Aureos typically consist of an N-terminal domain with unknown function, a basic region leucine zipper (bZIP) DNA-binding domain, and a C-terminal light-oxygen-voltage (LOV) sensing domain. LOV domains are a subgroup of the Per-Arnt-Sim (PAS) superfamily that sense blue light using a noncovalently bound flavin cofactor. Photon absorption of the flavin results in formation of a flavin-C4(a)-cysteinyl adduct with a conserved cysteine residue, which initiates a cascade of structural rearrangements within the LOV core that are propagated to the domain boundaries. Here, we present crystal structures of a fully light-adapted LOV dimer as well as of a dark state LOV monomer of PtAu1a.

To obtain the structure of a fully light-adapted PtAu1aLOV dimer, we set up crystallization screens of wildtype PtAu1aLOV under continuous blue light illumination and obtained colorless crystals overnight. Their lack of color is indicative of formation of the flavin-C4(a)-cysteinyl adduct. As expected from the MALS measurements, light-activated PtAu1aLOV crystallized as a dimer that features an assembly similar to other N-cap-comprising PAS dimers. The two PtAu1aLOV protomers are related by a 2-fold non-crystallographic symmetry that does not apply to the A´α helices. Analysis of the contact area using the PISA web server revealed a buried surface area (BSA) of 1524 Å2, which is similar to that observed for the VIVID light state dimer (1342 Å2), supporting the observed dimer arrangement as biologically relevant. The main dimerization interface is formed by a network of hydrophobic residues on the core β-sheet and A´α. Superposition of the dark and light state structures not only reveals a variety of light-induced side chain rearrangements, but also a significant change of the position of the A´α helix that is released from the hydrophobic patch on the LOV core, thus exposing the dimerization site. Compared with the dark state structure, the C-terminal part of Jα is unstructured and the hydrogen bonds between Gln365 and the carbonyl and amine group of Cys316 are broken, indicating light-induced Jα undocking from the LOV β-sheet and subsequent unfolding as suggested previously. The formation of the covalent Cys287–FMN adduct and the resulting doming of the isoalloxazine ring at position C4a are supported by the Fo-Fc omit map and the 2Fo-Fc map. Additionally, the highly conserved Tyr266 located on strand Bβ shows a light-induced rotation out of the dimer interface, which is prerequisite for LOV dimerization.

>GAMGDFSFIKALQTAQQNFVVTDPSLPDNPIVYASQGFLNLTGYSLDQILGRNCRFLQGPETDPKAVERIRKAIEQGNDMSVCLLNYRVDGTTFWNQFFIAALRDAGGNVTNFVGVQCKVSDQYAATVTKQQEEEEEAAANDDED[2x]>MSTSTSQIAVEYPIPVYRFIVSVGDEKIPFNSVSGLDISYDTIEYRDGVGNWFKMPGQSQSTNITLRKGVFPGKTELFDWINSIQLNQVEKKDITISLTNDAGTELLMTWNVSNAFPTSLTSPSFDATSNDIAVQEITLMADRVIMQAV[6x];>[6x]MENQILTQLYGRGWAFPPVFSLEKGVEMAEGAEDVRQSLQILFSTEPGERLMRENYGCGLNDFMFENIRNELIAEIESHIHDNVLRYEPRADMTDIQVRQSPGMGNTLQVQVMYRLRGSDINQQIQGVLALSEGRVTEVV;>[6x]MELNELTNKLSNLVPMTDFKLDNRASLQLLKYIEAYTKIIPFNSGDKYWNDFFFMSGNTPEKLAKLYQKEIEPNGELLPQQAFLLAVLRLLETPISLLNVLPAAHRELYYRELLGLSSHAAQPDQVALSMELNSTVMEQLLPEGTLFEAGQDEQGNALQYALDASLLANRGYISDLRWLRNDGEKQWVTSAPWDLQAQVSLPSDGIRLFGKTNSDQQVFGGVLITSSLLAMEAGIRKIIVTFEQEMNTQELVAQVSSGNQWLTLTSEVNKKEVTLTLSDKEPAISAPEDLDNLFFTQPVLRLQGKDSQALPEVTGISVSEKDDTKDTSFEMYHLTPFGYSSDIEPLEENPALYLGFTDVKPGQTLALYWKLKSPQQPTVSWYYLDQHNQWAELDSWVSDGTQNLYQDGTWHVELPVDASNQAEQMPVGRYWLRAVVEVPAHEGALGKAPWLYGLIYNAMTATLVNVDSISDSHFLTPLPASSIQRPVEPIIVLASVNQPWASWGGRIPESYSAFFERIAQNLSHRNRSLTWGNMVTLLKERYVSIFDVKYPGNDELTRVPALEQQQLTVIPANRYNDSDDSLRPVLNPARLQEMADWLQQKDSPWASIEVRNPEYLDVKIHYEVIFKPDVNEDFGYRQLQQQLCEVYMPWSIDEQRPVVLNNSINYFQLLATIQQQPLVERVTRLTLHRADSSDESDGTASVEAKDNEVLILVWEEDDNLQYRGNDYE;>[6x]MSNQDALFHSVKDDIHFDTLLEQAHQVIEKQAEKLWSDTAEHDPGITFLQGISYGVSDLAYRHTLPLKDLLTPAPDEQQQEGIFPAEFGPHNTLTCGPVTADDYRKALLDLHSSDSLDGTQQDEGDFLFRSVQLVREPEKQRYTYWYDATKREYSFVNSEGAKEFTLRGNYWLYLEPTRWTQGNIAAATRQLTEFLTKNRNIGESVSNIIWLQPVDLPLLLDVELDDDVGAQDVPGIFAAVYSTAEQYLMPGAQRYRTEVLQNAGMSNDQIFEGPLLEHGWIPELPAARDYTQRLTLNLSRLVNSLLEIEGIKHVNRLRLDDSFDKTAIEPVKGDTWSWSIKEGYYPRLWGEDPLNQLAQQNGPLRVIAKGGISVSVSKEQIQASLPSQSLIQNEPVILAYGQHRDVGSYYPVSDTLPPCYGLQHSLSESEHLLPLHQFMLPFEQLLACGCQQIAMLPRLLAFQREGYEVWGDQWPFKSGSVNDDAHQDYAPALKDLLGQIALDSDHELDIINYLLGYFGTQRAPRTFTTQLDDFRAVQQGYLAQQPTLTYHRSNIRIDQVSSLQKRIAARMGLGGELFKPQPDLSQLPFYLIEHRALLPVKPNSQFDKEQKPASVTEEGGSQTGQHYVVIEQKGIDGKLTQGQVINLILYEGEQGETQFTIRGQMVFKTEGDKFWLDVNNSAQLEYNLARVMTAAKASKLFWQNSPVWMEDMGYRLAYASDQSSLPVNQRRLTRTVQTPFPPMVVVGSEITLLKQVGIVNLKKAESEKLYAKVVSFDRIEGTLIIERLGNSTLAFPTSEEAWRYSWYFSGEKYERTDRFSFVISVVVNSDLIKLPGVDPYKLEEWVKETILTEFPAHISMIIHWMDREAFLNFANTYQRWQNNGTPLGDAAYSILESLTLGKLPSALKGVGTMRIATSSQREEVVGSNGDQWNTDGITQNELFYVPKES;>MERLQPGVTLTESIITMGQQEIPSAVPVFIGYTVRYPEQSEASVRIDSLAEYTSLFGDDHVMMFAVRHYFDNGGQQAFVLPLKDNMPSVEMTTAEAENLIAALRSATVSEAIGGHSQITLILVPDMARLNDSDIDDSSTQVSLWSQGWEALLQLSQVRPNLFVLLDAPDNVEQAQKCMTTLSSDYRQWGAAYWPRLETTYQKEISGKDNESQGIFQGTVLSPTAAVAAVIQRTDNDAGVWKAPANIALSQVIRPVKSYLQGSVLFNSSGTSLNVIRSFPGKGIRVWGCRTLENTDNTQWRYLQTRRLVSYVTAHLTQLARMYVFEPNNELTWMKLKGQSYNWLRQLWLQGGLYGSQEDEAFNILLGVNETMTEDDVRAGKMIMKVELAVLFPAEFIEISLVFNTQTEALS[6x];>[6x]MSLIERGLAKLTINAYKDREGKIRAGTLQAMYNPDSLQLDYQTDYQQSQAINSEKQSSIYVQAKPAGLSLELIFDATMPGNKTPIEEQLMQLKQLCSVDATSNETRFLQVKWGKMRWESRGYFAGRAKSLSVNYTLFDRDATPLRVRVILALVADESLVLQETEQNLQSPAKIALRIQDGVSLALMAASTASTLSGGVDYLTLAWQNGLDNLNGFVPGEILQATRGDES;>MTTVTSYPGVYIEELNSLALSVSNSATAVPVFAVDEQNQYISEDNAIRINSWMDYLNLIGNFNNEDKLDVSVRAYFANGGGYCYLVKTTSLEKIIPTLDDVTLLVAAGEDIKTTVDVLCQPGKGLFAVFDGPETELTINGAEEAKQAYTATPFAAVYYPWLKADWANIDIPPSA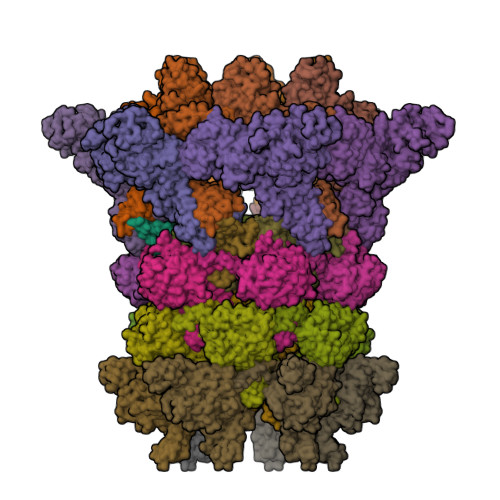VMAGVYASVDLSRGVWKAPANVALKGGLEPKFLVTDELQGEYNTGRAINMIRNFSNTGTTVWGARTLEDKDNWRYVPVRRLFNSVERDIKRAMSFAMFEPNNQPTWERVRAAISNYLYSLWQQGGLAGSKEEDAYFVQIGKGITMTQEQIDAGQMIVKVGLAAVRPAEFIILQFTQDVEQR[6x];>MNDYYTPVVSHRFMASFIFNRIPDPLDIRFQRISGLSRELQVTQYSEGGENARNNYLAEKIQHGTLTLERGVMTVSPLTWMFDRVLSGEKIAYADVVVMLLNENSLPLSSWTLSNALPVRWQTSDFDANSNAILVNTLELRYQDMRWLGVKI[6x];>[6x]MSAILKAPGVYIEEDASLALSVSNSATAVPVFIGKFTPTVVDSIQVCTRISNWLEFTSSFSLAPTVEIVVQSNTESESESETYHYIETINLSPAVEALRLYFQNGGGACYIYPLNDAEDELVLAAIPEVIEQKGDITLLVCPELDLDYKTKIYGAVSSLLNDNKVGYFLIADSNDGESVSGVWNSAKAAAYYPQLETNLKFSTLPGDKDIRISGYQDDDETHKPKNLDELRTINEALAQDIDARLLEEKQRAVIIPPSAAIAGIYCQTDNRRGVWKAPANVALTGIGSLLDKVDDERQGEMNDKGINVIRSFTDRGFMVWGARTCVDAANISWRYIPVRRLFNSVERDIRQALRAVLFETNSQPTWVRAKAAVDQYLYTLWQKNALMGARPEEAYFVQIGQDITMSEADIKQGKMIMTVGLAAVRPAEFIILQFTQDVVQ> MDSSTWSPKTTAVTRPVETHELIRNAADISIIVIYFVVVMAVGLWAMFSTNRGTVGGFFLAGRSMVWWPIGASLFASNIGSGHFVGLAGTGAASGIAIGGFEWNALVLVVVLGWLFVPIYIKAGVVTMPEYLRKRFGGQRIQVYLSLLSLLLYIFTKISADIFSGAIFINLALGLNLYLAIFLLLAITALYTITGGLAAVIYTDTLQTVIMLVGSLILTGFAFHEVGGYDAFMEKYMKAIPTIVSDGNTTFQEKCYTPRADSFHIFRDPLTGDLPWPGFIFGMSILTLWYWCTDQVIVQRCLSAKNMSHVKGGCILCGYLKLMPMFIMVMPGMISRILYTEKIACVVPSECEKYCGTKVGCTNIAYPTLVVELMPNGLRGLMLSVMLASLMSSLTSIFNSASTLFTMDIYAKVRKRASEKELMIAGRLFILVLIGISIAWVPIVQSAQSGQLFDYIQSITSYLGPPIAAVFLLAIFWKRVNEPGAFWGLILGLLIGISRMITEFAYGTGSCMEPSNCPTIICGVHYLYFAIILFAISFITIVVISLLTKPIPDVHLYRLCWSLRNSKEERIDLDAEEENIQEGPKETIEIETQVPEKKKGIFRRAYDLFCGLE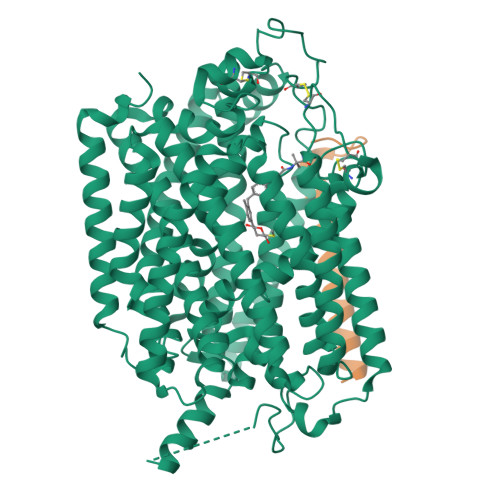QHGAPKMTEEEEKAMKMKMTDTSEKPLWRTVLNVNGIILVTVAVFCHAYFA;> MSALSLLILGLLMAVPPASCQQGLGNLQPWMQGLIAVAVFLVLVAIAFAVNHFWCQEEPEPAHMILTVGNKADGVLVGTDGRYSSMAASFRSSEHENAYENVPEEEGKVRSTPM> MFERFTEKAIKVIMLAQEEARRLGHNFVGTEQILLGLIGEGTGIAA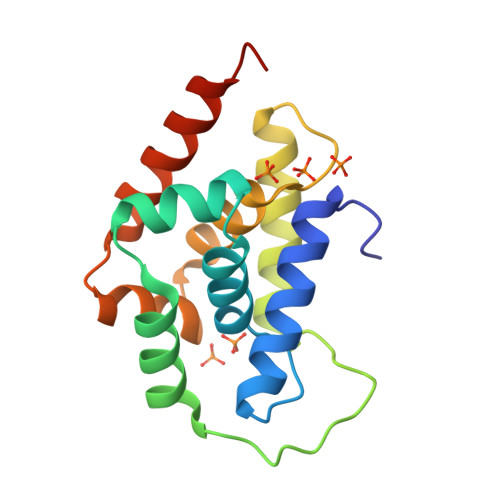KVLKSMGINLKDARVEVEKIIGRGSGFVAVEIPFTPRAKRVLELSLEEARQLGHNYIGSEHLLLGLLREGEGVAARVLENLGADPSNIRTQVIRMVGENLEHHHHHH The synthesis of inositol pyrophosphates is mediated in plants by two classes of ATP-grasp fold kinase: PPIP5 kinases, known as VIH, and members of the inositol tris/tetrakisphosphate kinase (ITPK) family, specifically ITPK1/2. A molecular explanation of the contribution of ITPK1/2 to inositol pyrophosphate synthesis and turnover in plants is incomplete: the absence of nucleotide in published crystal structures limits the explanation of phosphotransfer reactions, and little is known of the affinity of potential substrates and competitors for ITPK1. Herein, we describe a complex of ADP and StITPK1 at 2.26 Å resolution and use a simple fluorescence polarization approach to compare the affinity of binding of diverse inositol phosphates, inositol pyrophosphates, and analogues. By simple HPLC, we reveal the novel catalytic capability of ITPK1 for different inositol pyrophosphates and show Ins(3,4,5,6)P4 to be a potent inhibitor of the inositol pyrophosphate-synthesizing activity of ITPK1.

Refined against all data to 2.26 Å resolution, the final structural model had an R-factor of 19.0% (Rfree 24.1%). Relative to AtITPK4, ITPK1 possesses a “tether” insertion following the central subdomain, while AtITPK4 possesses a “tab” in the N-terminal subdomain. The tether comprises a polypeptide connection between the C-terminal β-strand of the central domain and a helix of the C-terminal domain running under the protein. This polypeptide lies across the top of the active site cavity, linking the two domains. In all the ITPK1s of known molecular structure where this polypeptide is resolved, it provides residues that contribute to the ATP cofactor/substrate binding pocket. Consistent with the absence of the resolved nucleotide, this region is disordered in the crystal structure of ZmITPK1,38 but in StITPK1, it is stabilized in most parts by adventitious interactions with a neighboring copy of the molecule in the crystal lattice. As for other ITPK1 enzymes, the active site of StITPK1 is narrow, unlike the more open active site in AtITPK4, and features a highly positively charged active site. However, due to the lack of bound nucleotide in the crystal structure of ZmITPK1, the central domain is displaced relative to that seen in the potato enzyme structure and InsP6 binds in such a way that in-line phosphoryl transfer from the γ-phosphate of ATP is implausible. On the other hand, in the pose of InsP6 predicted for StITPK1, InsP6 binds with its “receiving” 5-phosphate in the F-specificity subsite, contrasting with the “receiving” 1-hydroxyl of Ins(3,4,5,6)P4 which occupies subsite A. Again, polar contacts to the ligand are made by Q224 of the tether region; thus, the bound nucleotide may stabilize the central subdomain and a portion of the tether, enabling recognition of InsP6 and catalysis.

> GPMKMAEPMRRYSVGYALAPKKQASFIQVSLVNLAKERGIDLIKIDTDKPLIDQGPFDCVLHKMDGDDWKRQLKEYGSEFPQALIIDSPEAIERLHNRISMLQAVGEVEIDCENASFGIPKQTVIYDAKMVSAINLENEGLEFPVIAKPLVADGSAKSHKMLLVFNKDGLRKLKPPIVLQEFVNHGAVIFKVYVVGDYVKCVKRKSLPDVKEDGLGRLESYLPFSQVSNLNNFEKNDDKYYKLMNLENAEYPPLSFLTNIARGLRRVTKLHLFNFDVIRDDRVGNRYLIIDINYFPGYAKMPNYERVLTDFFWDVLNQNDKS Here, we report the crystal structure of the C-terminal hydrophilic domain of nsp4 (nsp4C) from MHV strain A59, together with the structure of a C425S site-directed mutant. The structure covers an 89 amino acid region from T408 to Q496 and is shown to possess a new fold. In particular, the C-terminal hydrophilic region from T408 to Q496 is highly conserved among all the coronaviruses, indicating that nsp4C may play a similar and conserved role in coronavirus replication.

Mutagenesis of Cys425 to Ser broke the disulfide bond, but two mutant monomers interact with each other via their cross-linked C-termini to form a strikingly different “close” conformation compared to the “open” conformation of the wild-type dimer, in which the C-termini of the wild-type monomers are oppositely oriented. Thus, the mutant C425S monomer structure contains four α-helices (α1–α4) and four β-strands (β1–β4). The conformation of the four α-helices and β-strands β1–β2 are identical to WT, while a short β-strand (β3, S449–M452) between α3 and α4 and a long β-strand β4 (β4, T487-S493) at the C-terminal are formed for stability of the dimer during the crystal packing. Two monomers of the mutant C425S also form a dimer in the asymmetric unit, with their N-termini in parallel and in the same orientation. The C-terminal β4 strands of the two monomers are cross-linked and form anti-parallel β-sheets together with β3 at the bottom of the dimer. Ser425 from each monomer in the mutant dimer is oriented on the outside of the dimer, far away from intersecting C-termini of the dimer. Thus, mutating Cys425 to Ser does not directly influence the interaction between the C-termini of these two monomers. In the case of the C425S mutant, the disulfide bond is dissociated and the dimer adopts a more stable conformation by crystal packing: the flexible C-termini of two monomers are stabilized by hydrogen bond interactions between the amino acids in the Ala488-Thr492 (β4) and Ser450-Met452 (β3) loops, which form stable anti-parallel β-sheets at the bottom of the dimer, resulting in clear electron density from residues Ser489-Leu495. The intersecting C-termini of the monomers result in a “closed” conformation of the mutant dimer. Thus the conformation of mutant C425S dimer is not likely to be physiological but instead an artifact of crystallization.

>[2x]GPLGSTFEEMALTTFMITKESYSKLKNSVSDVAFNRYLSLYNKYRYFSGKMDTAAYREAACSQLAKAMETFNHNNGNDVLYQPPTASVTTSFLQ>MTNTIDVYPGKDFGDDDPQYQQALKYDDLIAIQKQPWVASATPAVSQNLRLRYNNVDVAASANGVSGDYFNVYGMTFSEGNTFNQEQLNGRAQVVVLDSNTRRQLFPHKADVVGEVILVGNMPARVIGVAEEKQSMFGSSKVLRVWLPYSTMSGRVMGQS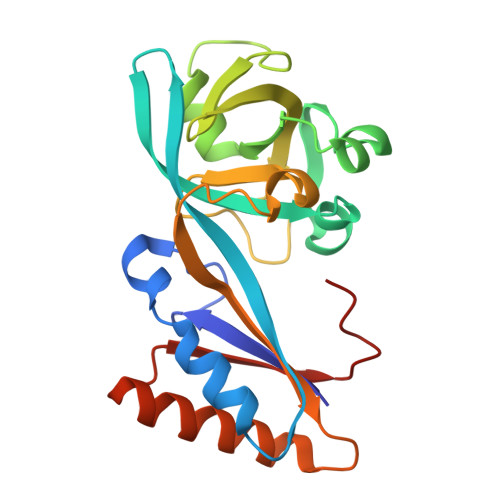WLNSITVRVKEGFDSAEAEQQLTRLLSLRHGKKDFFTWNMDLEHHHHHH[2x]>MKPIFSRGPS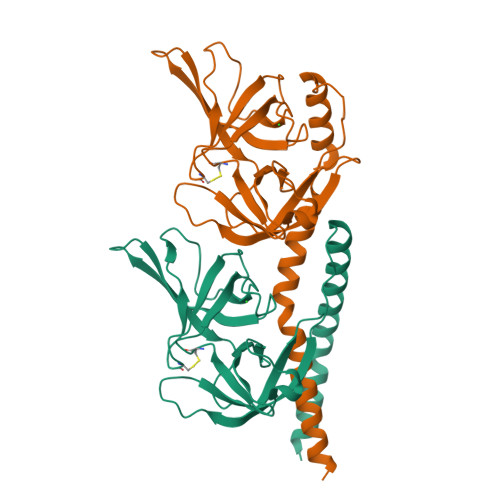LQIRLILAVLVALGIIIADSRLGTFSQIRTYMDTAVSPFYFVSNAPRELLDGVSQTLASRDQLELENRALRQELLLKNSELLMLGQYKQENARLRELLGSPLRQDEQKMVTQVISTVNDPYSDQVVIDKGSVNGVYEGQPVISDKGVVGQVVAVAKLTSRVLLICDATHALPIQVLRNDIRVIAAGNGCTDDLQLEHLPANTDIRVGDVLVTSGLGGRFPEGYPVAVVSSVKLDTQRAYTVIQARPTAGLQRLRYLLLLWGADRNGANPMTPEEVHRVANERLMQMMPQVLPSPDAMGPKLPEPATGIAQPTPQQPATGNAATAPAAPTQPAANRSPQRATPPQSGAQPPARAPGGQ[2x]> GSMGKALVIVESPAKAKTINKYLGSDYVVKSSVGHIRDLPTSGSAAKKSADSTSTKTAKKPKKDERGALVNRMGVDPWHNWEAHYEVLPGKEKVVS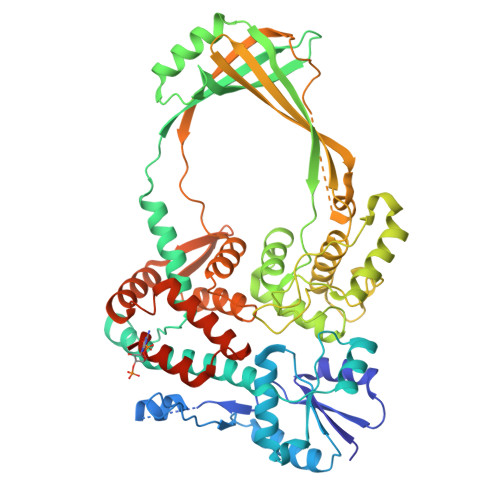ELKQLAEKADHIYLATDLDREGEAIAWHLREVIGGDDARYSRVVFNEITKNAIRQAFNKPGELNIDRVNAQQARRFMDRVVGYMVSPLLWKKIARGLSAGRVQSVAVRLVVEREREIKAFVPEEFWEVDASTTTPSGEALALQVTHQNDKPFRPVNKEQTQAAVSLLEKARYSVLEREDKPTTSKPGAPFITSTLQQAASTRLGFGVKKTMMMAQRLYEAGYITYMRTDSTNLSQDAVNMVRGYISDNFGKKYLPESPNQYASKENSQEAHEAIRPSDVNVMAESLKDMEADAQKLYQLIWRQFVACQMTPAKYDSTTLTVGAGDFRLKARGRILRFDGWTKVMPALRKGDEDRILPAVNKGDALTLVELTPAQHFTKPPARFSEASLVKELEKRGIGRPSTYASIISTIQDRGYVRVENRRFYAEKMGEIVTDRLEENFRELMNYDFTAQMENSLDQVANHEAEWKAVLDHFFSDFTQQLDKAEKDPEEGGMRPNQMVLTSI>PSLSKEAALVHEALVARGLETPLRPPVHEMDNETRKSLIAGHMTEIMQLLNLDLADDSLMETPHRIAKMYVDEIFSGLDYANFPKITLIENKMKVDEMVTVRDITLTSTSEHHFVTIDGKATVAYIPKDSVIGLSKINRIVQFFAQRPQVQERL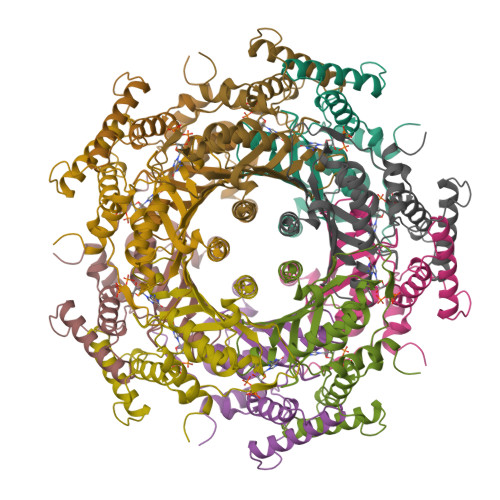TQQILIALQTLLGTNNVAVSIDAVHYCVKARGIRDATSATTTTSLGGLFKSSQNTRHEFLRAVRHHN[15x]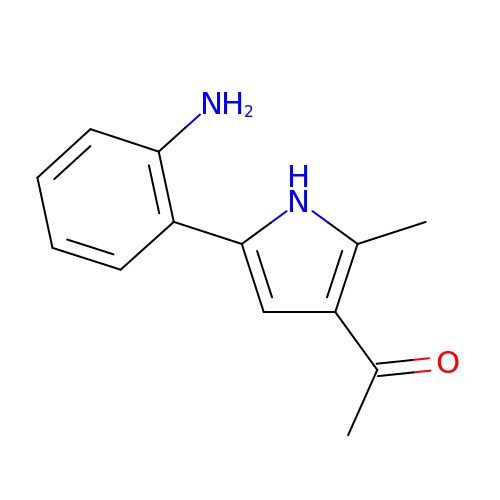1-[5-(2-aminophenyl)-2-methyl-1H-pyrrol-3-yl]ethan-1-one | C13 H14 N2 O | WSWGBAXEVIRMAC-UHFFFAOYSA-N>MSYQNLVSEAGLTQKHLIHGDKELFQHEMKTIFARNWLFLTHDSLIPSPGDYVTAKMGLDEVIVSRQNDGSVRAFLNVCRHRGKTIVHAEAGNAKGFVCNYHGWGYGTNGELQSVPFEKELYGDAIKKKCLGLKEVPRIESFHGFIYGCFDAEAPPLIDYLGDAAWYMEPTFKHSGGLELVGPPGKVVVKANWKTFAENFVGDIYHVGWTHASILRVGQSVFTPLAGNAMLPPEGSGLQMTSKYGSGMSLMWDYYAGNHSADLVPDLMAFGGAKQEKLAKEIGDVRARIYRSHLNGTIFPNNSFLTGSAAFKVWNPIDENTTEVWTYAFVEKDMPEDLKRRLADAVQRTVGPGGYWESDDNDNMETLSQNAKKYQSSNSDLIASLGFGKDVYGDECYPGVVGPSGASETSYRGFYRAYQAHISSSNWAEFENASRNWHTELTKTTD[3x];>[3x]MMINTQEDKLVSAHDAEEFHRFYIVQDDALLQEVNTLLTREAHLLDIQAYKAWL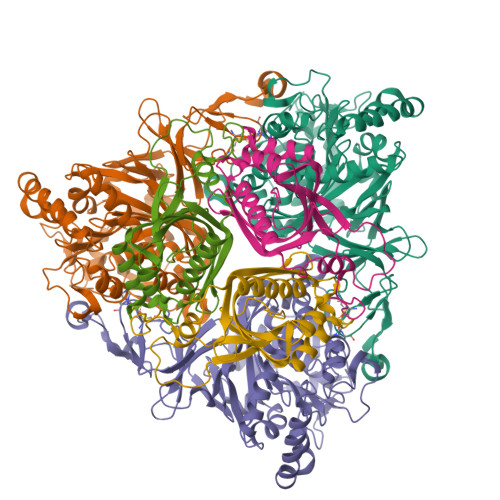EHCVAPEIKYQVISRELRSTSERRYQLNDAVNIYNENYQQLKVRVEHQMDPQNWPNSPKIRFTRFVTNVTAAKDKSAPEMLHVRSNLILHRARRGNEVDVFYATREDKWKRIEGGGIQLVERFVDYPERILPHNLLVFL>[2x]GSHMATFLIKHKASGKFLHPKGGSSNPANDTNLVLHSDIHERMYFQFDVVDERWGYIKHAASGKIVHPLGGKADPPNETKLVLHQDRHDRALFAMDFFNDNIIHKAGKYVHPKGGSTNPPNETLTVMHGDKHGAMEFIFVSPKNKDKRVLVYV

MytiLec, a lectin isolated from the Mediterranean mussel Mytilus galloprovincialis, was identified through a study of marine organisms and their adaptation to different habitats and environmental systems, and shown to bind α-D-galactose and N-acetyl-α-D-galactosamine (α-GalNAc). The structure is well ordered, with the entire main-chain of each monomer visible in the 2mFo-DFc electron density map, revealing a β-trefoil fold consisting of three related sub-domains. MytiLec is somewhat unusual in binding ligand at each subdomain, and it forms a dimer in solution, giving a total of six ligand sites per protein.

In order to understand how MytiLec binds to galactose and GalNAc, and whether the acetyl group contacts the protein, co-crystals of MytiLec and GalNAc were grown. These crystals, in space-group C2, diffracted to slightly higher resolution than the apo crystals, and also had a dimer in the asymmetric unit showing identical interactions between partner chains. Six GalNAc molecules were identified in the electron density map, and were sufficiently ordered for the electron density map to show a large hole in the centre of each ring. The very high-resolution diffraction data allowed the GalNAc ligands to be placed unambiguously at three sites per polypeptide, related by the pseudo-symmetry of the protein sequence. The principal side-chain contacts made by MytiLec with GalNAc are all charged, with the ligand cradled by three histidines and two carboxyl groups. Five hydrogen bonds form between the protein and each of the six ligand molecules. A HxDxH motif is found in each sub-domain, the first histidine (His 32, His 80 or His 124) lying against the sugar ligand but making no hydrogen bond with it. The axially positioned O4 atom makes two hydrogen bonds to histidine residues, the first residue of the HPxGG motif and the last one of the HxDxH motif. D-glucose differs from D-galactose only in the position of this epimeric oxygen, so the structure implies strong selectivity for galactose over glucose. The C2-N-acetyl group of the ligand points away from the protein and makes no significant contact with it, indicating that galactose will bind as well as GalNAc with the same binding mode.>GSHMESFLLSKVSFVIKKIRLEKGMTQEDLAYKSNLDRTYISGIERNSANLTIKSLELIMKGLEVSDVVF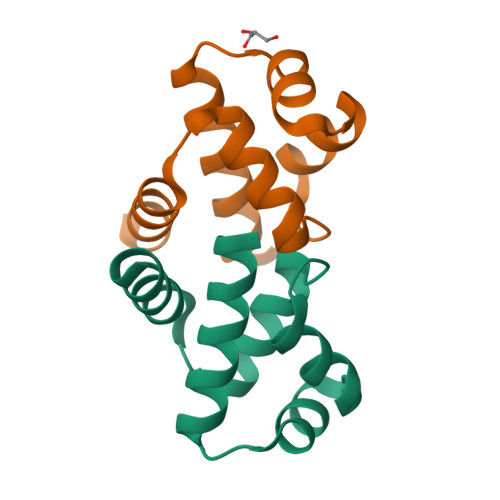FEMLIKEILKHD[4x]>[2x]GHDASFLNAVVKVYCTHTAPDYSLPWQKQRQFTSTGSAF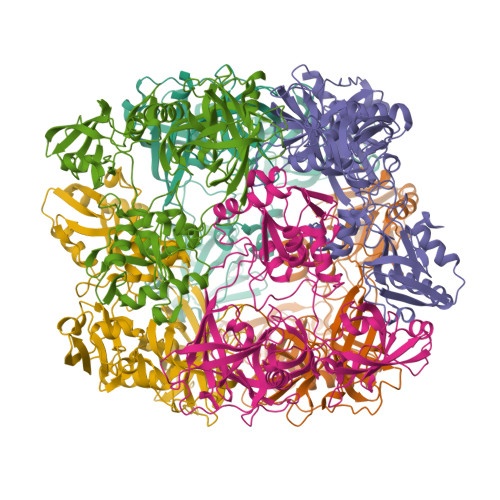MIGDGKLLTNAHCVEHDTQVKVKRRGDDRKYVAKVLVRGVDCDIALLSVESEDFWKGAEPLRLGHLPRLQDSVTVVGYPLGGDTISVTKGVVSRIEVTSYAHGSSDLLGIQIDAAINPGNSGGPAFNDQGECIGVAFQVYRSEETENIGYVIPTTVVSHFLTDYERNGKYTGFPVLGIEWQKMENPDLRKSMGMESHQKGVRIRRIEPTAPESQVLKPSDIILSFDGVNIANDGTVPFRHGERIGFSYLISQKYTGDSALVKVLRNKEILEFNIKLAIHKRLIPAHISGKPPSYFIVAGFVFTTVSVPYLRSEYGKEYEFDAPVKLLEKHLHAMAQSVDEQLVVVSQVLVSDINIGYEEIVNTQVVAFNGKPVKNLKGLAGMVENCEDEYMKFNLDYDQIVVLDTKTAKEATLDILTTHCIPSAMSDDLKTEERN>ETGKIFCKSVSKDPDFRLKQIDYVIPVQQDRSICMNNPLLDISDGFFTYIHYEGINSCKKSDSFKVLLSHGEIVDRGDYRPSLYLLSSHYHPYSMQVINCVPVTCNQSSFVFCHISNNTKTLDNSDYSSDEYYITYFNGIDRPKTKKIPINNMTADNRYIHFTFSGGGGVCLGEEFIIPVTTVINTDVFTHDYCESFNCSVQTGKSLKEICSESLRSPTNSSRYNLNGIMIISQNNMTDFKIQLNGITYNKLSFGSPGRLSKTLGQVLYYQSSMSWDTYLKAGFVEKWKPFTPNWMNNTVISRPNQGNCPRYHKCPEICYGGTYNDIAPLDLGKDMYVSVILDSDQLAENPEITVFNSTTILYKERVSKDELNTRSTTTSCFLFLDEPWCISVLETNRFNGKSIRPEIYSYKIPKYCGTKHHHHHH[5x];>[5x]ETGAKNLEPVSWSSLNPKFLSGKGLVIYPKIGDKLDIICPRAEAGRPYEYYKLYLVRPEQAAACSTVLDPNVLVTCNRPEQEIRFTIKFQEFSPNYMGLEFKKHHDYYITSTSNGSLEGLENREGGVCRTRTMKIIMKVGQDGTKHHHHH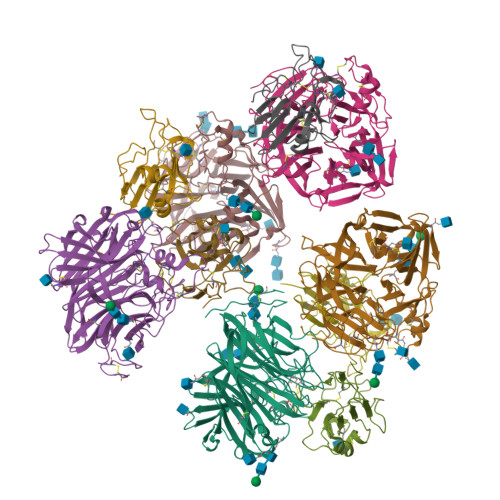H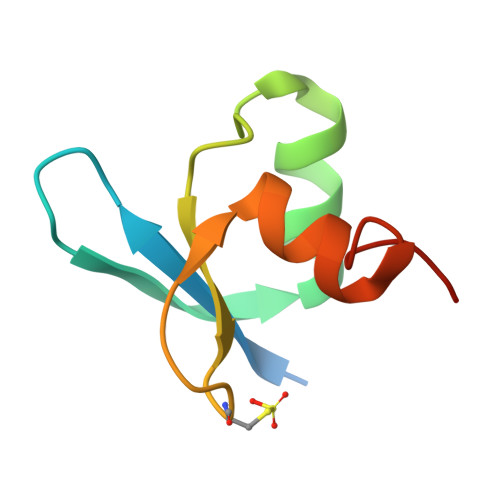> GPLESHGAARKWFYKDPQGEIQGPFTTQEMAEWFQAGYFSMSLLVKRGCDEGFQPLGEVIKMWGRVPFAPGPS>[2x]SVPIVSAWEKGMEAARALMDKYHVDNDLKANFKLLPDQVEALAAVCKTWLNEEHRGLQLTFTSNKTFVTMMGRFLQAYLQSFAEVTYKHHEPTGCALWLHRCAEIEGELKCLHGSIMI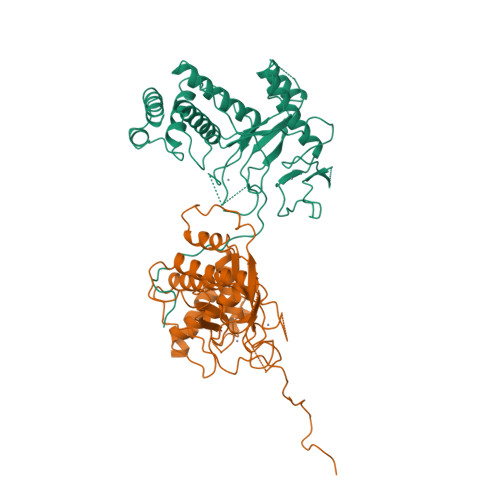NKEHVIEMDVTSENGQRALKEQSSKAKIVKNRWGRNVVQISNTDARCCVHDAACPANQFSGKSCGMFFSEGAKAQVAFKQIKAFMQALYPNAQTGHGHLLMPLRCECNSKPGHAPFLGRQLPKLTPFALSNAEDLDADLISDKSVLASVHHPALIVFQCCNPVYRNSRAQGGGPNCDFKISAPDLLNALVMVRSLWSENFTELPRMVVPEFKWSTKHQYRNVSLPVAHSDARQNPFDF>[4x]MVSLEKNDHLMLARQLPLKSVALILAGG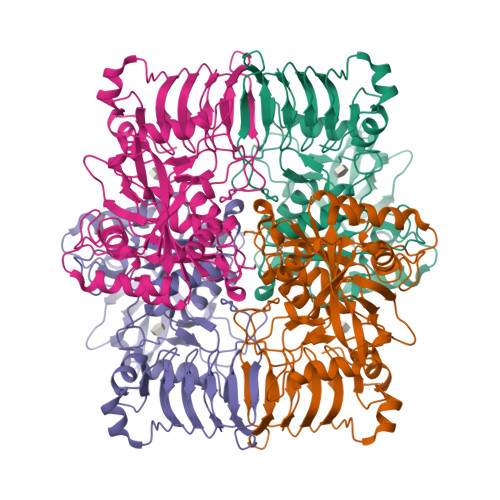RGTRLKDLTNKRAKPAVHFGGKFRIIDFALSNCINSGIRRMGVITQYQSHTLVQHIQRGWSFFNEEMNEFVDLLPAQQRMKGENWYRGTADAVTQNLDIIRRYKAEYVVILAGDHIYKQDYSRMLIDHVEKGARCTVACMPVPIEEASAFGVMAVDENDKIIEFVEKPANPPSMPNDPSKSLASMGIYVFDADYLYELLEEDDRDENSSHDFGKDLIPKITEAGLAYAHPFPLSCVQSDPDAEPYWRDVGTLEAYWKANLDLASVVPELDMYDRNWPIRTYNESLPPAKFVQDRSGSHGMTLNSLVSGGCVISGSVVVQSVLFSRVRVNSFCNIDSAVLLPEVWVGRSCRLRRCVIDRACVIPEGMVIGENAEEDARRFYRSEEGIVLVTREMLRKLGHKQER>MSKKLLFQFDTDATPSVFDVVVGYDGGADHITGYGNVTPDNVGAYVDGTIYTRGGKEKQSTAIFVGGGDMAAGERVFEAVKKRFFGPFRVSCMLDSNGSNTTAAAGVALVVKAAGGSVKGKKAVVLAGTGPVGMRSAALLAGEGAEVVLCGRKLDKAQAAADSVNKRFKVNVTAAETADDASRAEAVKGAHFVFTAGAIGLELLPQAAWQNESSIEIVADYNAQPPLGIGGIDATDKGKEYGGKRAFGALGIGGLKLKLHR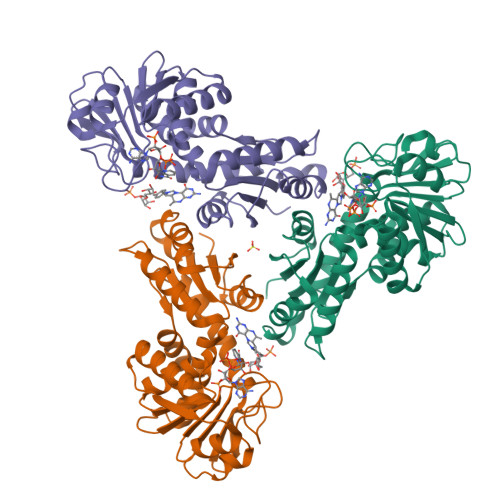ACIAKLFESSEGVFDAEEIYKLAKEMA[24x]>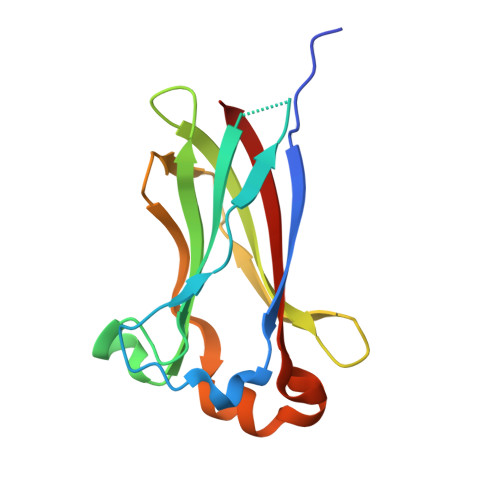 GSGGSGKVVKFSYMWTINNFSFCREEMGEVIKSSTFSSGANDKLKWCLRVNPKGLDEESKDYLSLYLLLVSCPKSEVRAKFKFSILNAKGEETKAMESQRAYRFVQGKDWGFKKFIRRDFLLDEANGLLPDDKLTLFCEVSVVQD> AYTTAQLVTAYTNANLGKAPDAATTLTLDAYATQTQTGGLSDAAALTNTLKLVNSTTAVAIQTYQFFTGVAPSAAGLDFLVDSTTNTNDLNDAYYSKFAQENRFINFSINLATGAGAGATAFAAAYTGVSYAQTVATAYDKIIGNAVATAAGVDVAAAVAFLSRQANIDYL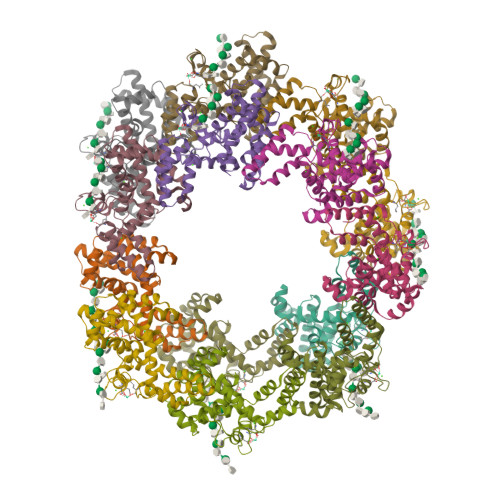TAFVRANTPFTAAADIDLAVKAALIGTILNAATVSGIGGYATATAAMINDLSDGALSTDNAAGVNLFTAYPSSGVSGSENLYFQ>MQYKKIITSESVGAGHPDKICDQISDAILDECLSQDQNSRVACEVLACNRLIVIAGEITTHAYVDVVKTAWEIIKPLGYDENDFTIISNVNKQSVDIAQSVDKTNKNLIGAGDQGIVFGYACDETPQYMPLTSVLAHELLKEIERQRRSKEFIKIQADMKSQVSIDYSNSTPLIETMLVSIQHDEDYDVEYFNKKVSAIMEQIAKKYNLNTNFKKIINSSGRFVIGGPIGDTGLTGRKIIVDTYGGVGHHGGGAFSGKDPTKVDRSASYFARWIAKNVVAAKLAKQCEIQLAFAI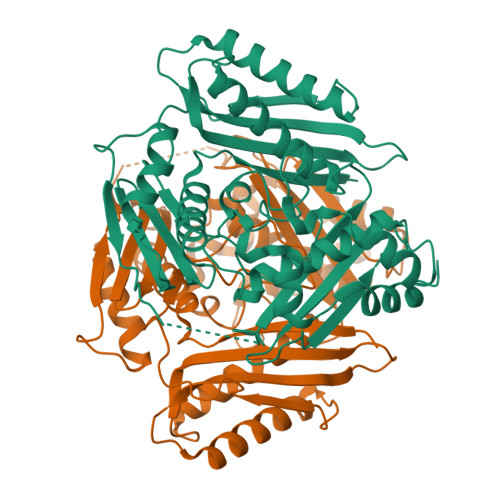GQPQPVAMYVNTFNTNLIDETKIFEAIKKSFNFDIKTFINDLNLWTTKYLPVATYGHFGRDDLDLSWEKLNKVEDLIKNSKH[4x]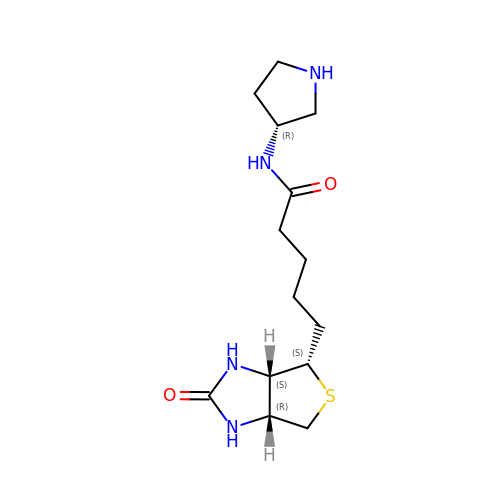5-[(3~{a}~{S},4~{S},6~{a}~{R})-2-oxidanylidene-1,3,3~{a},4,6,6~{a}-hexahydrothieno[3,4-d]imidazol-4-yl]-~{N}-[(3~{R})-pyrrolidin-3-yl]pentanamide | C14 H24 N4 O2 S | QSMYOZNFIUDGEL-BLFANLJRSA-N>[30x]MAHIFVKPELVAEIGVKQLQREIVLPGLVWTNPLTDFGGSKNDTITVRVPAITTANRRDLRDP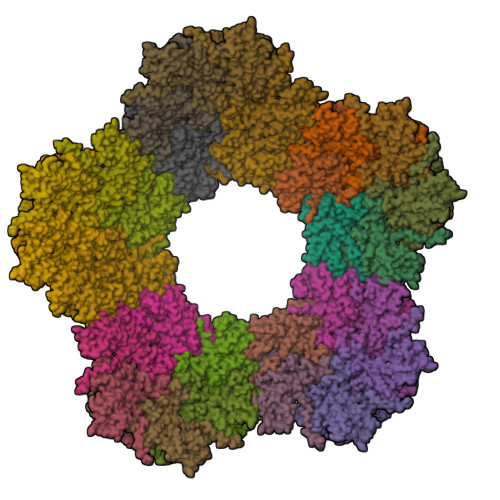DRTVIASELVEHSFGVTLDKHVYAALKFTDEQRTLDIRDYTKQVLMPQVSAVAYELEDYIAELIEGAPYEETILIDPADTVPAFITADQRMGEANVPTDSRRLVVGSAVAAALAKDKQFRHADWSGDQANAALREAHVGRLAGMNVIRSNAIAPDKAYLWHRTAFILAYRTPVVPEGAKAGASFSANGVALRWLADYDYSQLGDRTLLDVFTGRKVVTEVDGSFVRAVELQLQASSITIVGGAFALATTTGTKQLKVRDDNGTDVTARCTFASSAGTKATVSAAGLVTGVAAGTADITASYVPPQGGTAKTATVTVTVP Hda1 is a typical class II histone deacetylase from Saccharomyces cerevisiae. Two related proteins Hda2 and Hda3 are essential for the activity of Hda1 both in vivo and in vitro. Together, they form the yeast Hda1 HDAC complex, which specifically deacetylates H2B and H3, with Hda1 homo-dimer as the catalytic subunit and Hda2-Hda3 hetero-dimer as the non-catalytic subunit. Hda1 contains an N-terminal catalytic HDAC domain and a C-terminal ARB2 domain. The ARB2 domain is defined by sequence homology to the Arb2 protein, which is a subunit of the yeast Argonaute complex and is essential for histone H3 Lys9 (H3-K9) methylation, heterochromatin assembly, and siRNA generation.

To gain insight into the role of the C-terminal non-catalytic domain of Hda1 functioning in the deacetylation process, we determined the crystal structure of ARB2 domain of Hda1. The structure was solved by the SAD method using the Se anomalous signal. The final model has been refined to 2.7 Å resolution and the details of the data collection and refinement statistics are summarized in Table 1. There is one ARB2 domain molecule observed in the crystal asymmetric unit. The ARB2 domain adopts an α/β sandwich architecture with an arm protruding outside. The core structure comprises an eight-stranded β-sheet (β1↑-β2↓-β4↑-β3↑-β5↑-β6↑-β7↑-β8↑), flanked by three α-helices on the proximal side (α1, α3 and α8) and four α-helices on the distal side (α4, α5, α6 and α7). The protruded arm region spans residues 509–532, and contains a short α-helix (α2). Further examination of symmetry-related molecules indicates that two ARB2 domain molecules form a homodimer. As shown in Fig. 2A,B two symmetry-related ARB2 domain molecules come together to form an inverse “V” shape via the respective arm region. Residues Ile512, Ile523 and Leu525 located in the protruded arm region of each molecules form a hydrophobic core, which dominates the domain-domain interaction. The ITC results show that all of these mutants could weaken the interaction between the ARB2 domain and histones, suggesting that the inverse “V” shape groove is indeed involved in interacting with histones and the residues His604, His608 and Arg609 are indispensable for binding to H3-H4.

> HHHHHHGSMLQKAIRQQQQHYLSDEFNFVTLPLVSMDLPDNTVLCTPNISESNTIIIVVHDTSDIWAKRNVISGTIDLSSSVIIDNSLDFIKWGLDRKYGIIDVNIPLTLFEPDNYSGMITSQEVLIYLWDNYIKYFPSVAKIAFIGIGDSYSGIVHLLGHRDTRAVTKTVINFLGDKQLKPLVPLVDETLSEWYFKNSLIFSNNSHQCWKENESRKPRKKFGRVLRCDTDGLNNIIEERFEEATDFILDS> SLSAAQKDNVTSSWAKASAAWGTAGPEFFMALFDAHDDVFAKFSGLFSGAAKGTVKNTPEMAAQAQSFKGLVSNWVDNLDNAGALEGQCKTFAANHKAR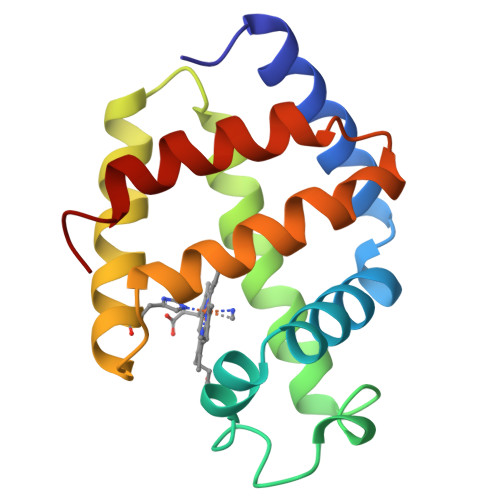GISAGQLEAAFKVLSGFMKSYGGDEGAWTAVAGALMGEIEPNM6-CHLORO-3-(3-METHYLISOXAZOL-5-YL)-4-PHENYLQUINOLIN-2(1H)-ONE | C19 H13 Cl N2 O2 | 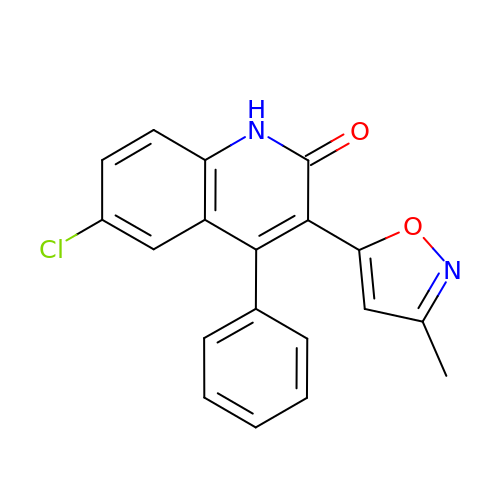QINNOQKHPLWGBK-UHFFFAOYSA-N>[4x]MAHGNEKATVLARLDELERFCRAVFLAVGTDEETADAATRAMMHGTRLGVDSH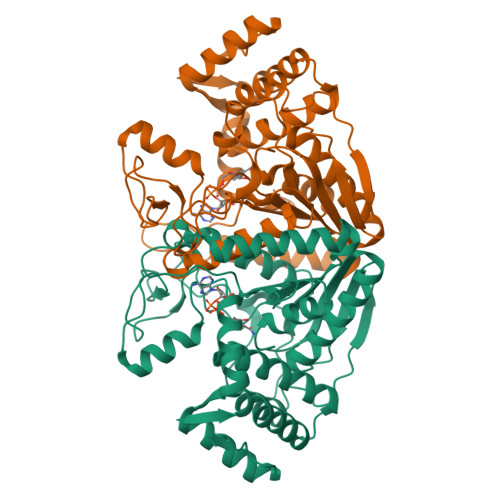GVRLLAHYVTALEGGRLNRRPQISRVSGFGAVETIDADHAHGARATYAAMENAMALAEKFGIGAVAIRNSSHFGPAGAYALEAARQGYIGLAFCNSDSFVRLHDGAMRFHGTNPIAVGVPAADDMPWLLDMATSAVPYNRVLLYRSLGQQLPQGVASDGDGVDTRDPNAVEMLAPVGGEFGFKGAALAGVVEIFSAVLTGMRLSFDLAPMGGPDFSTPRGLGAFVLALKPEAFLERDVFDESMKRYLEVLRGSPAREDCKVMAPGDREWAVAAKREREGAPVDPVTRAAFSELAEKFSVSPPTYH>KHSLPDLPYDYGALEPHINAQIMQLHHSKHHAAFVNNLNVTEEKYQEALAKGDVTAQIALQPALKFNGGGHINHSIFWTNLSPNGGGEPKGELLEAIKRDFGSFDKFKEKLTAASVGVQGSGWGWLGFNK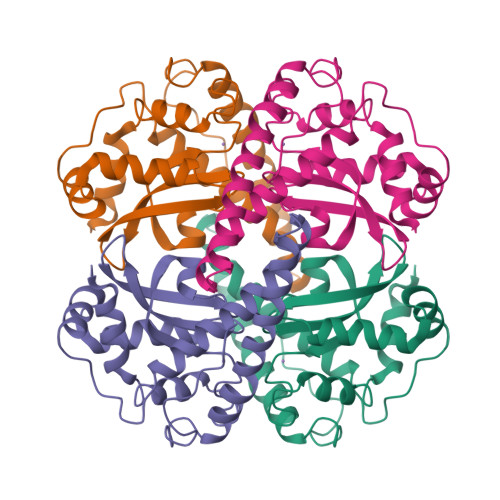ERGHLQIAACPNQDPLQGTTGLIPLLGIDVWEHAYYLQYKNVRPDYLKAIWNVINWENVTERYMACKK[2x]> GMTALRQDIDPNGLLEYSVVYTDRALNHMSKAFQEVMNDLLSNLKTVYNAEAAVIIPGSGTYGMEAVARQLTIDEDCLIIRNGWFSYRWTQILEKGKF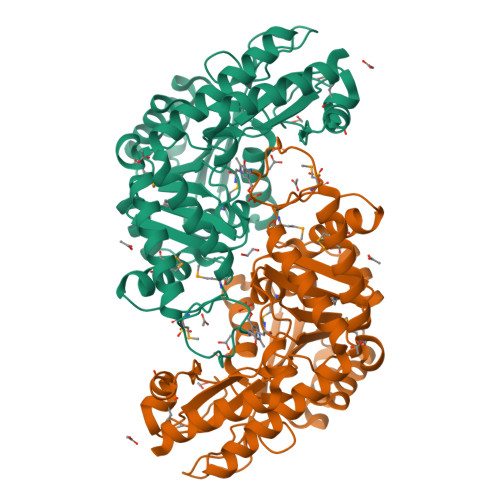AKSSTVLTAERTEDTEAPKPFAPVDIETAVAKIKEDKSAIVYAPHVETSSGIILSEEYIKALSEAVHSVGGLLVIDCIASGCVWLDMKELGIDVLISAPQKGWSSTPCAGLVMLSAAAIKKVESTESNCFSLDLKQWLTIMRAYENGGHAYHATMPTDSLRQFRDAILEAKEIGFDILRDAQWELGNRVRKVLTDKGIESVAAEGFEAPGVVVSYTERDDMHKGSAFAEAGLQIAAGVPLKVGEPDNFKTFRLGLFGLDKLTDIDGTVERFEKALDEVLAK> MNFFEYCISTYAKIFEETMNAVGDERVSQKKAIRDTMISAMREFPNVEAAEIWKAVYSAHMDRKSGIADPDIIQKVISAENSWKKSSGHAFEEMIKLLGNSSLEEYGMRILLQKDLNMMIENQEIANEPRDINWLKEQISSNVFDLYITVR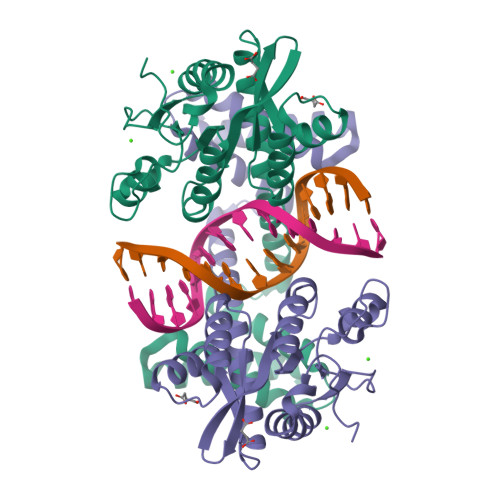NNDKEYVFGCIQSKTSIRDRVTRDREPSMKAMEAFFWSVAICLDGDFLKMPKFIAMVNGGTSNYRLNGWHGMYVFWDKPTIDRIYPIDINLELFVQHAREAAEDWLHRRQWFNYEWKAGQK>PFLELDTNLPANRVPAGLEKRLCAAAASILGKPADRVNVTVRPGLAMALSGSTEPCAQLSISSIGVVGTAEDNRSHSAHFFEFLTKELALG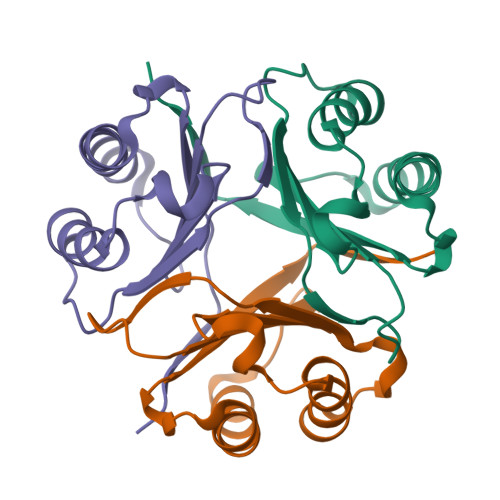QDRILIRFFPLESWQIGKIGTV[12x]>MRNKPGKATGKGKPVNNKWLNNAGKDLGSPVPDRIANKLRDKEFKSFDDFRKKFWEEVSKDP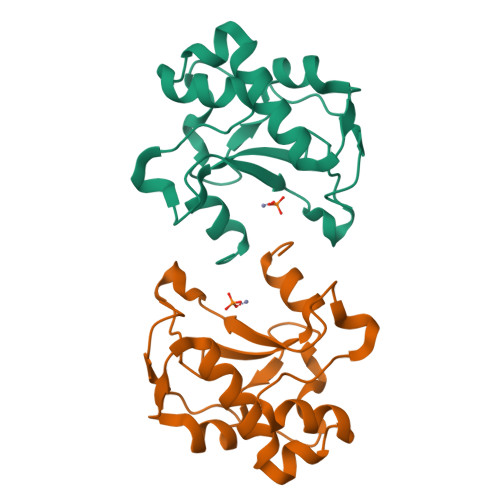ELSKQFSRNNNDRMKVGKAPKTRTQDVSGKRTSFELHHEKPISQNGGVYDMDNISVVTPKRHIDIHRGK[2x]> GPLGSEEDVPENNGILISIKEVINAEFSRDGTIHSSELKGVLELRINDHDLSHSNLKLADSIDVRDKSFQFKTHPNIDKQSFLS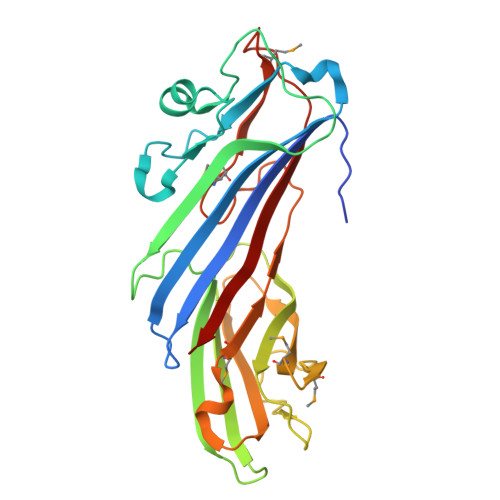TKLISLRDKSKAFPANDQSLGVLRWRKVAPAEDDSLIPLTLTTAVSPSESQQGFDVIIEYESVLETELADVIFTIPVFPQEPVDINTESSTCSDAEVVNMDQEMGTSIKISKIAANDAGALAFTIEAPYEDALYPMTVSFQESTRDKLAKSFTGMAIQSVVMANDHDQELPYDVITSLKSDEYLVQ3-{[(3R)-7,9-diamino-3-methyl-2,3-dihydrofuro[2,3-f]quinazolin-4-yl]oxy}benzonitrile 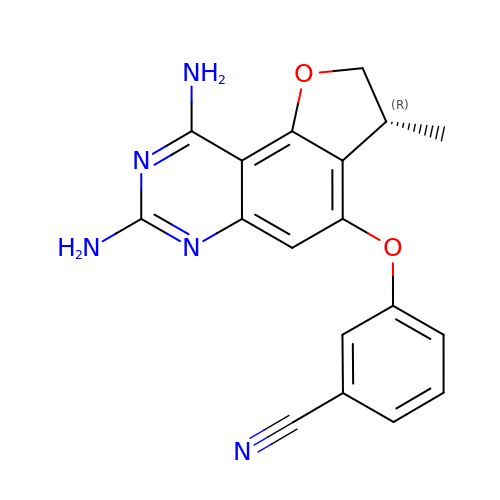| C18 H15 N5 O2 | XWYWWNRDHWMQAL-VIFPVBQESA-N7-(3,5-dimethoxyphenyl)-N-[(3S)-1-methylpiperidin-3-yl]-4-propanoyl-2,3,4,5-tetrahydro-1,4-benzoxazepine-9-carboxamide | C27 H35 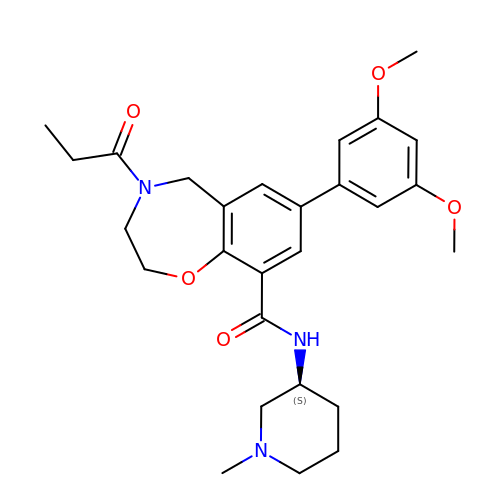N3 O5 | CUJLWYCUPPPASA-NRFANRHFSA-N> AEQKTLHIYNWTEYIAPDTVANFEKETGIKVVYDVFDSNEVLEGKLMAGSTGFDLVVPSAYFLERQLTAGVFQPLDKSKLPEWKNLDPELLKLVAKHDPDNKFAMPYMWATTGIGYNVDKVKAVLGENAPVDSWDLILKPENLEKLKSCGVSFLDDPEEVFATVLNYLGKDPNSTKADDYTGPATDLLLKLRPNIRYFHSSQYINDLANGDICVAIGWAGSVWQASNRAKEAKNGVNVSFSIPKEGAMAWFDVFAMPADAKNKDEAYQFLNYLLRPDVVAHISDHVFYANANKAATPLV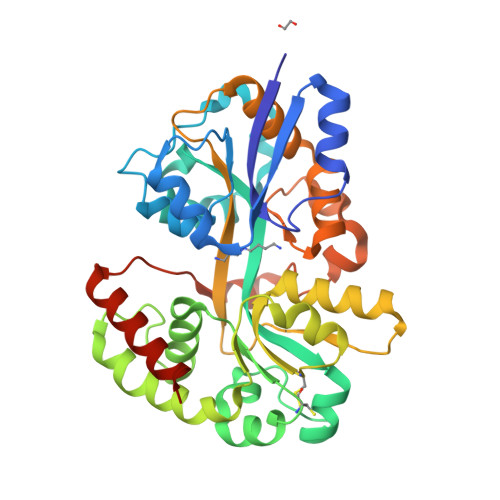SAEVRENPGIYPPADVRAKLFTQKVQDPKIDRVRTRAWTKVKSGKLEHHHHHH>[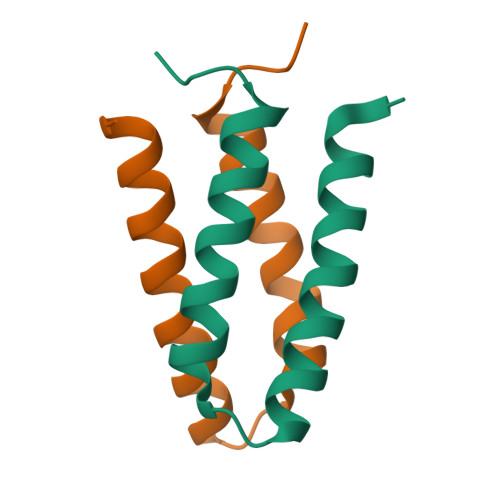6x]SKRLHLDDEKSSNLGEMVRVGEGKYREDFQMDEGEDPNLLFQSYLDNVGVQIVRQMRSGERFLKIWSQTVEEIVSYVTVNFPNPPRRSSEDKSTQTTGRELKKETTSAFSQRESQPSKA Here we studied 30 congeneric ligands that each present a distinct heteroarene for stacking between tyrosine residues at the dimer interface of procaspase-6. Complex X-ray crystal structures of 10 analogs showed that stacking geometries were well conserved, while high-accuracy computations showed that heteroarene stacking energy was well correlated with predicted overall ligand binding energies. Here we employed a congeneric set of molecular glues for procaspase-6 to study diverse heteroarene stacking on tyrosine side chains under physiologically relevant conditions. As a model system, this protein–ligand interaction exhibits desirable features such as a shape-persistent binding site, a conserved ligand binding mode across diverse analogs, and the positioning of the probe heteroarene at the terminus of the ligand structure.

To confirm that binding poses and stacking interactions were conserved across analogs 1–30, we solved procaspase-6 complex crystal structures for 10 representative analogs spanning 3 orders of magnitude in measured KD value. Importantly, all 10 structures revealed binding poses almost exactly analogous to that adopted by 1, with the probe heterocycles positioned in apparently productive stacking interactions with tyrosine 198A and 198B. The significantly improved KD values in the progression from pyridine to isosteric diazenes (1–4) and finally to triazene 25, for example, was fully consistent with guidelines from the Stahl2 and Wheeler16 groups that increasing numbers of heteroatoms lead to more favorable stacking with aromatic amino acid side chains.

>[4x]MSSASGLRRGHPAGGEENMTETDAFYKREMFDPAEKYKMDHRRRGIALIFNHERFFWHLTLPERRGTCADRDNLTRRFSDLGFEVKCFNDLKAEELLLKIHEVSTVSHADADCFVCVFLSHGEGNHIYAYDAKIEIQTLTGLFKGDKCHSLVGKPKIFIIQAARGNQHDVPVIPLDVVDNQTEKLDTNITEVDAASVYTLPAGADFLMCYSVAEGYYSHRETVNGSWYIQDLCEMLGKYGSSLEFTELLTLVNRKVSQRRVDFCKDPSAIGKKQVPCFASMLTKKLHFFPKSNENLYFQ> WSHPQFEKGATGRTTIAIDPVTRIEGHLKAEVVVENGKVVDARLSGGMYRGFETILRGR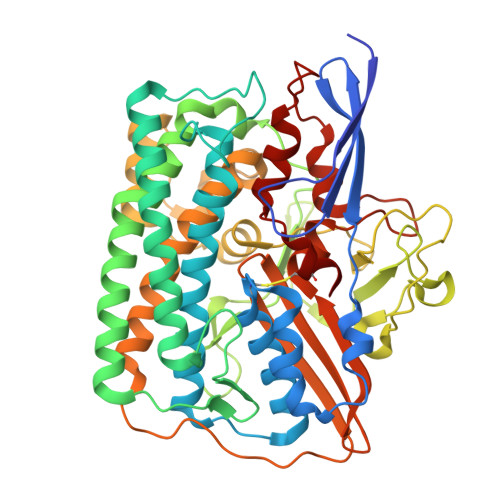DPRDASQIVQRICGVCPTAHSTASVLALDEAFGAKVPNNGRITRNLIFGANYLQSHILHFYHLSAQDFVQGPDTAPFVPRFPKSDLRLSKELNKAGVDQYIEALEVRRICHEMVALFGGRMPHVQGQVVGGATEIPTKEKLVEYAARFKKVRDFVEQKYVPVVYTIGSKYKDMFKVGQGFKAALCVGAFPLDNSGKKHLFMPGVYAKGKDMPFDPSKIKEYVKYSWFAEETTGLNYKEGKTIPAPDKAGAYSFVKAPRYDGLSLEVGPLARMWVNNPELSPVGKKLLKDLFGISAKKFRDLGEEAAFSLMGRHVARAEETYYMLGAIEGWLKEIKAGEDTVVMPAVPASAEGTGFTEAPRGSLLHYVKVKDSKIDNYQIVSASLWNCNPRDDMGQRGAVEEALIGIPVDDIQNPVNVARLIRAFDPULACAVH> MKMEYLQSEEKKDAINKQIHKKEEKEEKEIKIKRKNKVKQRIQIINQIKKYIEAKQQKKQIQSKNQRKYKGRMINTRKQVFKCLWGAQPAYNFSRIINHLRGDPVYQDNTKDVSLRGTFLRGKYDDLPTMIFFTEACDLTANWIPFFTNPQYDILAHRNVWLLNPRNFGNSDRHPSFDLQEMSDDVMRFMYSQKISMATLGGHGIGGKIALAVGCYHAER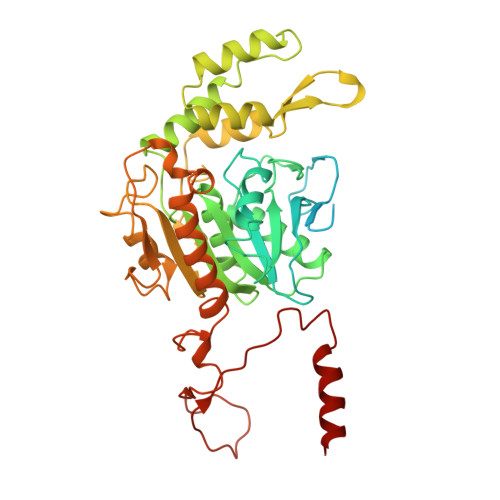VTGVFSIDSSPMDQRYHEAFKEFKGYVNALTEINFKTWSDKDVKVFLKENIKDPKWRSIFTNNISKNAKTQSDSFNFEINYLNHNLNFNKADSLGNWAVKNGIYTGRAHFIFPEYSRWVHLATNTLPMHKVCARVKGFGHDIFYVQGDENPLNHWVYDFENYANVVASKLNKFLHSYDGVHALLKDRTEIGNFMIPDRIKSRNDSKHIYGDYSPAHLHHNWRFNHIYEKHDELDKKLNEQ>MSSSVPTVKLFIGGKFVESKSDKWIDIHNPATNEVIGRVPQATKAEMDAAIASCKRAFPAWADTSVLSRQQVLLRYQQLIKENLKEIAKLITLEQGKTLADAEGDVFRGLQVVEHACSVTSLMMGETMPSITKDMDLYSYRLPLGVCAGIAPFNFPAMIPLWMFPMAMVCGNTFLMKPSERVPGATMLLAKLLQDSGAPDGTLNIIHGQHEAVNFICDHPDIKAISFVGYNKAGEYIFERGSRHGKRVQANMGAKNHGVVMPDANKENTLNQLVGAAFGAAGQRCMALSTAVLVGEAKKWLPELVEHAKNLRVNAGDQPGADLGPLITPQAKERVCNLIDSGTKEGASILLDGRKIKVKGYENGNFVGPTIISNVKPNMTCY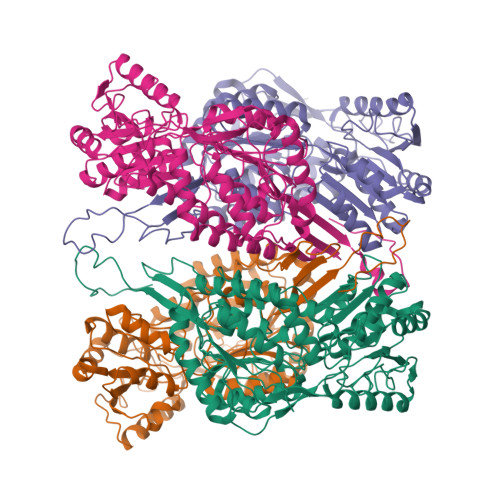KEEIFGPVLVVLETETLDEAIQIVNNNPYGNGTAIFTTNGATARKYAHLVDVGQVGVNVPIPVPLPMFSFTGSRSSFRGDTNFYGKQGIQFYTQLKTITSQWKEEDATLSSPAVVMPTMGRENLYFQ[4x]> GPGSMSKRLRSSDVCADCNGPDPSWASVNRGTFICDE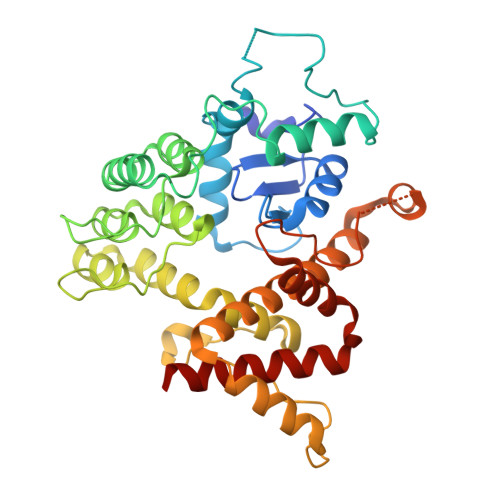CCSVHRSLGRHISQVRHLKHTAWPPTLLQMVETLYNNGANSIWEHSLLDPASIMSGRRKANPQDKVHPNKAEFIRAKYQMLAFVHRLPCREDDSVTAKDLSKQLHSSVRTGNLETCLRLLSLGAQANFFHPEKGSTPLHVASKAGQILQAELLAVYGADPGTQDSSGKTPVDYARQGGHHELAERLIEIQYELTDRLAFYLCGRKPDHKSGQHFLIPQRADAALDLSELAKAAKKKLQSLSNHLFEELAMDVYDEVDRRETDAVWLATQNHSTLVTETTVVPFLPVNPEYSSTRNQGRQKLARFNAHEFATLVIDILSDAKRRQQGS> MGIVNVPNCNTTKYQQLARTAVAIYNYHEQAHLTFVENLNCKEQLGEGDYYYITLAATDDAGKKAI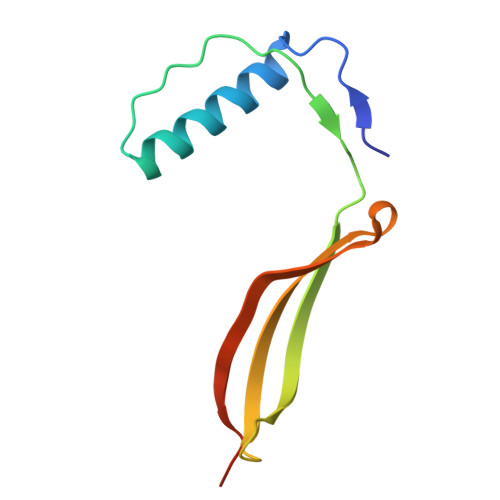YEAKIGVVESAGWTGVEEFKLVGSLEHHHHHH>[3x]KKAVPYNRMKLMIVGNTGSGKTTLLQQLMKTKKSDLGMQSATVGIDVKDWPIQIRDKRKRDLVLNVWDFAGREEFYSTHPHFMTQRALYLAVYDLSKGQAEVDAMKPWLFNIKARASSSPVILVGTHLDVSDEKQRKACMSKITKELLNKRGFPAIRDYHFVNATEESDALAKLRKTIINESLNFKIRDQLVVGQLIPDCYVELEKIILSERKNVPIEFPVIDRKRLLQLVRENQLQLDENELPHAVHFLNESGVLLHFQDPALQLSDLYFVEPKWLCKIMAQILTVKVEGCPKHPKGIISRRDVEKFLSKKRKFPKNYMSQYFKLLEKFQIALPIGEEYLLVPSSLSDHRPVIELPHCENSEIIIRLYEMPYFPMGFWSRLINRLLEISPYMLSGRERALRPNRMYWRQGIYLNWSPEAYCLVGSEVLDNHPESFLKITVPSCRKGCILLGQVVDHIDSLMEEWFPGLLEIDICGEGETLLKKWALYSFNDGEEHQKILLDDLMKKAEEGDLLVNPDQPRLTIPISQIAPDLILADLPRNIMLNNDELEFEQAPEFLLGDGSFGSVYRAAYEGEEVAVKIFNKHTSLRLLRQELVVLCHLHHPSLISLLAAGIRPRMLVMELASKGSLDRLLQQDKASLTRTLQHRIALHVADGLRYLHSAMIIYRD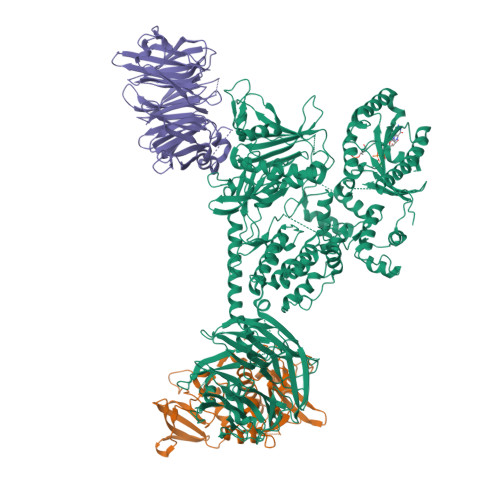LKPHNVLLFTLYPNAAIIAKIADYGIAQYCCRMGIKTSEGTPGFRAPEVARGNVIYNQQADVYSFGLLLYDILTTGGRIVEGLKFPNEFDELEIQGKLPDPVKEYGCAPWPMVEKLIKQCLKENPQERPTSAQVFDILNSAELVCLTRRILLPKNVIVECMVATHHNSRNASIWLGCGHTDRGQLSFLDLNTEGYTSEEVADSRILCLALVHLPVEKESWIVSGTQSGTLLVINTEDGKKRHTLEKMTDSVTCLYCNSFSKQSKQKNFLLVGTADGKLAIFEDKTVKLKGAAPLKILNIGNVSTPLMCLSESTNSTERNVMWGGCGTKIFSFSNDFTIQKLIETRTSQLFSYAAFSDSNIITVVVDTALYIAKQNSPVVEVWDKKTEKLCGLIDCVHFLREVMVKENKESKHKMSYSGRVKTLCLQKNTALWIGTGGGHILLLDLSTRRLIRVIYNFCNSVRVMMTAQLGSLKNVMLVLGYNRKNTEGTQKQKEIQSCLTVWDINLPHEVQNLEKHIEVRKELAEKMRRTSVE>GPGSKPFTLPILTIGELSNSRFPAPIDELYTSPNEGLVVQPQNGRSTLDGELLGTTQLVPSNICSLRGRINAHLPDNQHRWNMQVTNANGTPFDPTEDVPAPLGTPDFLANIYGVTSQRNPDNTCRAHDGILATWSPKFTPKLGSVVLG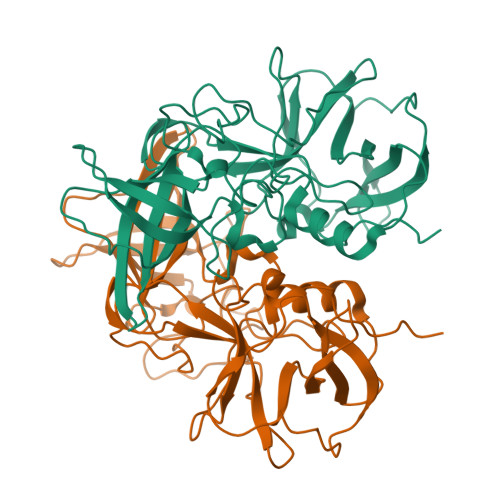TWEDRDFDINQPTRFTPVGLYDTDHFNQWALPNYSGALTLNMNLAPSVAPLFPGEQLLFFRSHIPLKGGTSNGAIDCLLPQEWVQHFYQESAPSSTDVALIRYTNPDTGRVLFEAKLHRQGFITVANSGSRPIVVPPNGYFRFDSWVNQFYSLAPM[2x]> GSALTVRDWPALEALAKTMPADAGARAMTDDDLRAAGVDRRVPEQKLGAAIDEFASLRLPDRIDGRFVDGRRANLTVFDDARVAVRGHARAQRNLLERLETELLGGTLDTAGDEGGIQPDPILQGLVDVIGQGKSDIDAYATIVEGLTKYFQSVADVMSKLQDYISAKDDKNMKIDGGKIKALIQQVIDHLPTMQLPKGADIARWRKELGDAVSISDSGVVTINPDKLIKMRDSLPPDGTVWDTARYQAWNT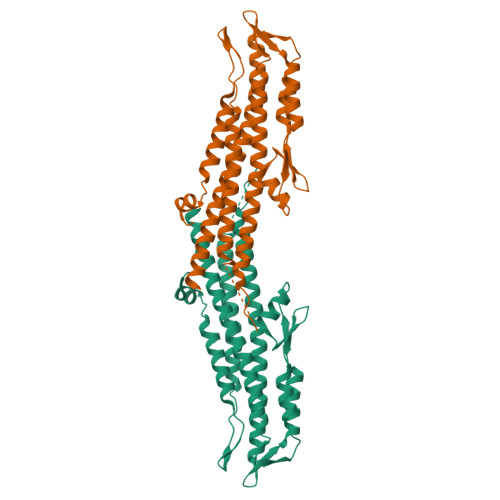AFSGQKDNIQNDVQTLVEKYSHQNSNFDNLVKVLSGAISTLTDTAKSYLQI>[2x]SIKSEFAEGAAVFVEGVAVFLTMMAAFQNGDKEAVAQYLARGASLYTRHEELLNRLLQKLRREGNKEAVTLMNEFTATFQTGKSLANALIAAFKNGDDDSFE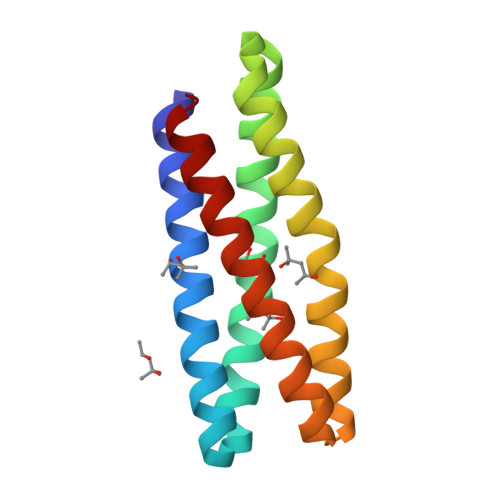SYLQAIWKVIAKMATILDQIAKAI> MSGTFHGDGHAPMSPFEDTFQFEDNSSNEDTHIAPTHFDDGATSNKYSRPQVSFNDETPKNKREDAEEFTFNDDTEYDNHSFQPTPKLNNGSGTFDDVELDNDSGEPHTNYDGMKRFRMGTKRNKKGNPIMGRSKTLKWARKNIPNPFEDFTKDDIDPGAINRAQELRTVYYNMPLPKDMIDEEGNPIMQYPRNKIRTTKYTPLTFLPKNILFQFHNFANVYFLVLIILGAFQIFGVTNPGLSAVPLVVIVIITAIKDAIEDSRRTVLDLEVNNTKTHILEGVENENVSTDNISLWRRFKKANSRLLFKFIQYCKEHLTEEGKKKRMQRKRHELRVQKTVGTSGPRSSLDSIDSYRVSADYGRPSLDYDNLEQGAGEANIVDRSLPPRTDCKFAKNYWKGVKVGDIVRIHNNDEIPADIILLSTSDTDGACYVETKNLDGETNLKVRQSLKCTNTIRTSKDIARTKFWIESEGPHSNLYTYQGNMKWRNLADGEIRNEPITINNVLLRGCTLRNTKWAMGVVMFTGGDTKIMLNSGITPTKKSRISRELNFSVVINFVLLFILCFVSGIANGVYYDKKGRSRFSYEFGTIAGSAATNGFVSFWVAVILYQSLVPISLYISVEIIKTAQAAFIYGDVLLYNAKLDYPCTPKSWNISDDLGQVEYIFSDKTGTLTQNVMEFKKCTINGVSYGRAYTEALAGLRKRQGIDVETEGRREKAEIAKDRDTMIDELRALSGNSQFYPEEVTFVSKEFVRDLKGASGEVQQRCCEHFMLALALCHSVLVEANPDNPKKLDLKAQSPDEAALVATARDVGFSFVGKTKKGLIIEMQGIQKEFEILNILEFNSSRKRMSCIVKIPGLNPGDEPRALLICKGADSIIYSRLSRQSGSNSEAILEKTALHLEQYATEGLRTLCIAQRELSWSEYEKWNEKYDIAAASLANREDELEVVADSIERELILLGGTAIEDRLQDGVPDCIELLAEAGIKLWVLTGDKVETAINIGFSCNLLNNEMELLVIKTTGDDVKEFGSEPSEIVDALLSKYLKEYFNLTGSEEEIFEAKKDHEFPKGNYAIVIDGDALKLALYGEDIRRKFLLLCKNCRAVLCCRVSPSQKAAVVKLVKDSLDVMTLAIGDGSNDVAMIQSADVGIGIAGEEGRQAVMCSDYAIGQFRYLARLVLVHGRWSYKRLAEMIPEFFYKNMIFALALFWYGIYNDFDGSYLYEYTYMMFYNLAFTSLPVIFLGILDQDVNDTISLVVPQLYRVGILRKEWNQRKFLWYMLDGLYQSIICFFFPYLVYHKNMIVTSNGLGLDHRYFVGVYVTTIAVISCNTYVLLHQYRWDWFSGLFIALSCLVVFAWTGIWSSAIASREFFKAAARIYGAPSFWAVFFVAVLFCLLPRFTYDSFQKFFYPTDVEIVREMWQHGHFDHYPPGYDPTDPNRPKVTKAGQHGEKIIEGIALSDNLGGSNYSRDSVVTEEIPMTFMHGEDGSPSGYQKQETWMTSPKETQDLLQSPQFQQAQTFGRGPSTNVRSSLDRTREQMIATNQLDNRYSVERARTSLDLPGVTNAASLIGTQQNN;> MVNFDLGQVGEVFRRKDKGAIVSGDNPEEEEDVDASEFEEDEVKPVRTKNRRPKEDAFTQQRLAAINPVLTPRTVLPLYLLIAVVFVIVGGCILAQNSKVDEVTIYYQDCMTNATSSWSDIPSEHWQFVFHKYKTYNTAPQWRFVDDESDDFTKQRGTCQIRFTTPSDMKNNVYLNYVLEKFAANHRRYVLSFSEDQIRGEDASYETVHDATGINCKPLSKNADGKIYYPCGLIANSMFNDTFPLQLTNVGDTSNNYSLTNKGINWESDKKRYKKTKYNYTQIAPPPYWEKMYPDGYNETNIPDIQDWEEFQNWMRPGAFDKITKLIRINKNDTLPAGEYQLDIGLHWPVLEFNGKKGIYLTHGSHLGGRNPFLGIVYLIGGCICAAMALILLTFWLFGGRKIADASSLSWNMK

P4 ATPases are involved in phospholipid translocation: they flip lipids from the extracellular side of the plasma membrane or from the lumenal side of internal organelles to the cytosolic side. Most P4 ATPases function as a heterodimeric complex: a catalytic α-subunit containing 10 transmembrane α-helices (TMHs) and a regulatory β-subunit of the Cdc50 (cell division cycle 50) protein family containing two TMHs. Dnf1 and Dnf2 share the same β-subunit, Lem3, and both are also capable of transporting PE and GlcCer. Here, we report the cryo-EM structures of Dnf1–Lem3 in three different states (E1, E1P-ADP, and E2P) and Dnf2–Lem3 in five different states (E1, E1-ATP, E1P-ADP, E2P, and E2P-transition).

There were Dnf1–Lem3 in the E1 (apo), E1P-ADP (AlF4−-ADP), and E2P (BeF3−) states; and Dnf2–Lem3 in the E1 (apo), E1-ATP (AMPPCP), E1P-ADP (ADP-AlF4−), E2P-transition (AlF4−), and E2P (BeF3−) states. By comparing the 3D maps of Dnf1–Lem3 and Dnf2–Lem3 in the E1, E1P-ADP, and E2P states, which were the three states observed for both flippases, we found that the structures were superimposable in all three states. In the E1 state, the A domain moves toward the membrane bilayer and becomes separated from the N domain. Due to the lack of interaction, the A and N domains are flexible and are visible in the 3D maps only at a low display threshold. However, there is a unique helix-turn-helix motif (E692-S737) in the N domain of Dnf1 and Dnf2 that is absent in Drs2 and ATP8A1. In the E1 state, the helix-turn-helix interacts with the P domain, specifically, its Lys-702 and Arg-703 interacting with the P domain Glu-994, Asn-998, and Asn-1008. Finally, the Dnf1 and Dnf2 switch back to the E1 state by auto-dephosphorylation. During this switch, the A and N domains become flexible again, and the TMH1-2 tilt back to narrow and close the exoplasmic substrate-binding site and open the cytosolic substrate-binding site. It is during this last transition that PL1 in the exoplasmic site is forced to flip and enter the cytosolic substrate site, replacing the resident PL2 there and leading to the release of PL2 from the flippases.>SELNEKLATAWEGFTKGDWQNEVNVRDFIQKNYTPYEGDESFLAGATEATTTLWDKVMEGVKLENRTHAPVDFDTAVASTITSHDAGYINKQLEKIVGLQTEAPLKRALIPFGGIKMIEGSCKAYNRELDPMIKKIFTEYRKTHNQGVFDVYTPDILRCRKSGVLTGLPDAYGRGRIIGDYRRVALYGIDYLMKDKLAQFTSLQADLENGVNLEQTIRLREEIAEQHRALGQMKEMAAKYGYDISGPATNAQEAIQWTYFGYLAAVKSQNGAAMSFGRTSTFLDVYIERDLKAGKITEQEAQEMVDHLVMKLRMVRFLRTPEYDELFSGDPIWATESIGGMGLDGRTLVTKNSFRFLNTLYTMGPSPEPNMTILWSEKLPLNFKKFAAKVSIDTSSLQYENDDLMRPDFNNDDYAIACCVSPMIVGKQMQFFGARANLAKTMLYAINGGVDEKLKMQVGPKSEPIKGDVLNYDEVMERMDHFMDWLAKQYITALNIIHYMHDKYSYEASLMALHDRDVIRTMACGIAGLSVAADSLSAIKYAKVKPIRDED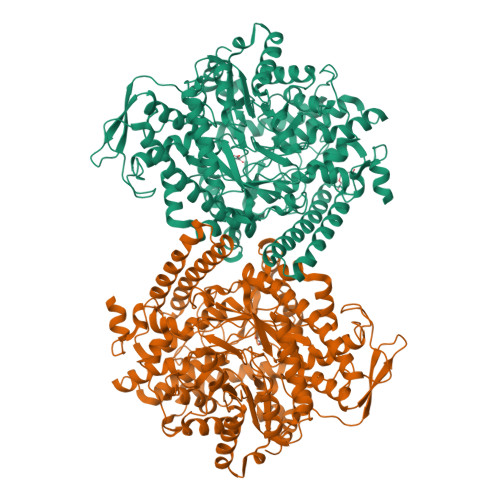GLAIDFEIEGEYPQFGNNDPRVDDLAVDLVERFMKKIQKLHTYRDAIPTQSVLTITSNVVYGKKTGNTPDGRRAGAPFGPGANPMHGRDQKGAVASLTSVAKLPFAYAKDGISYTFSIVPNALGKDDEVRKTNLAGLMDGYFHHEASIEGGQHLNVNVMNREMLLDAMENPEKYPQLTIRVSGYAVRFNSLTKEQQQDVITRTFTQSM[2x]> GSHMANPLAPYTLPQIATKVQVKHVPGKGRCLYTKHDLEPGSIIFVETPVLVAIPSLDEELWSVLTEINDEEALELPPVWHLAAICSLTMLDDEKKKICLDKWVPDPDRAPSDDVLRVINRAGLQVHPKLYERMLMVWRYNSFGHHTEQHGLVLYNRISMMAHSCRATACWHYGEDDAFILRARVKLQAGDELTISYIGDDDLFKSTNVRREKVYGWLFTCQCVRCAAPVDNARGFRCPLCGTGAMFFKTEDGETTSSACTICQAFPTQET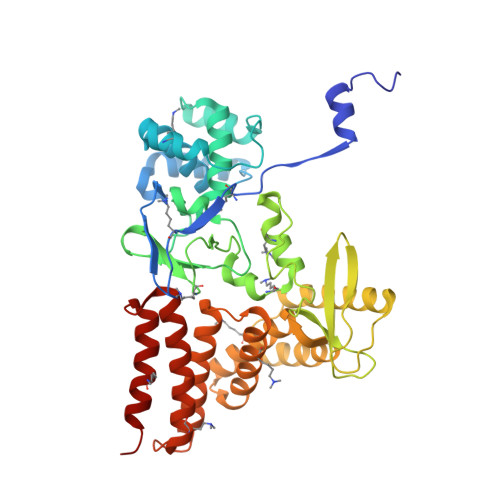IQEYLDFEQAYVDRLAETDKSDVPDAELVYNQATRVFAQHWVLYQLHTILFEGYRDAGNSESASFHQMERIKYVSQVMPLASYTLAWLYEEMGDTMLNKAEESGPEVPAHKLNVISRHFEDAYNLLYILCGEDHDYTVAAGTKKTACEERLPA> CPFPEPK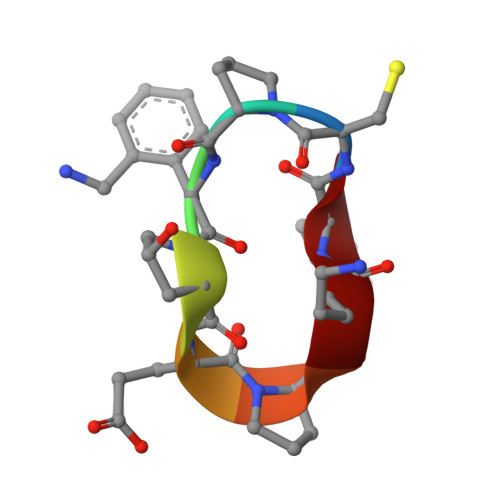L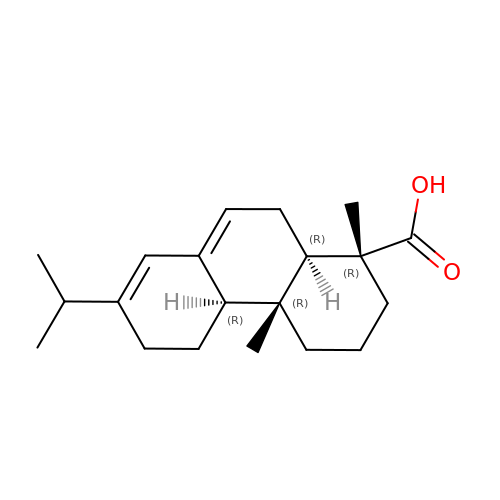Abietic acid | C20 H30 O2 | RSWGJHLUYNHPMX-ONCXSQPRSA-N>[2x]MKLHERLRELRSERGLRLKDVAEVAQISVPYLSDLERGRTNPSLETLQTLAG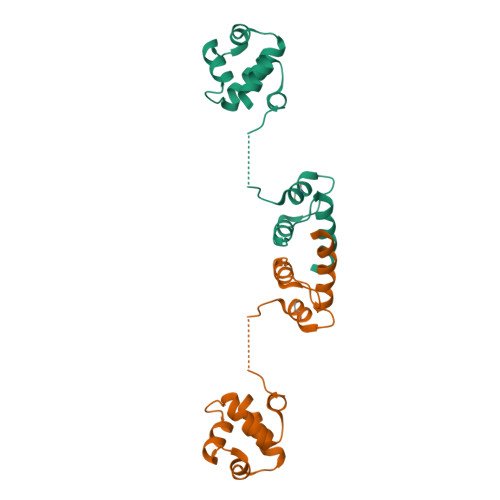AYNITVHDLLEGVEFYGMSTEGALPKGLSDLMADPTLGPQITPDWVRTLSRIELRGKRPRDKQDWYEIYLHLKRILS>[2x]MQAPTLGAAANFALFTTAGAVTNTGLSHITGDVGTNNAASTNFGNVDGVMQDSNGATSAAAADLLIAYNLLNAAIPTATLAPLLGNGTTLTAGNYFIGQGASLSGTLTLDGGGNSNSVFIFKIQGALSSAANTQVLLTNGALACNVFWKVEGLVDLATNTVMKGNVVA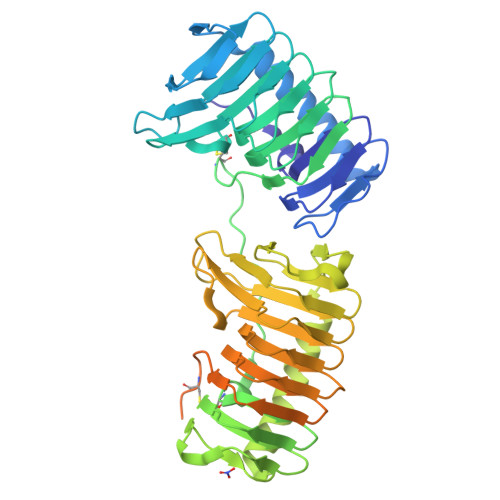NNAAIVLQSGVSLEGRALSTTGAITVTGVTVRKPILCGSAVLTGPVAPNLGTVVCYTIFSGNGALTNAGITYVTGDVGTNVGLTTGFQADNVNGTIHSNPDTSTAQAALDLNNAYTYLNTLPTDIELLYPAAFGQNLVLTPHTYLLNAATVLNGKVTLDAQGNENAVFVIKINGALSTTVNASVELINGAIAKNVFWKVDGAVDLNDYTKFKGSVIGNNGAVIINTGVEIEGRVLSTSGGISTFGINAQMTPGCELLGTGSNTVAIQAAKFYPNPFSSVLNVTMEDLNGGSTLTIYNAAGSQVFSKVLSTKTTSLSMKLPAGVYFYQMIGKNGAKQAGKLIAKPHHHHHH CARBIDOPA | C10 H14 N2 O4 | 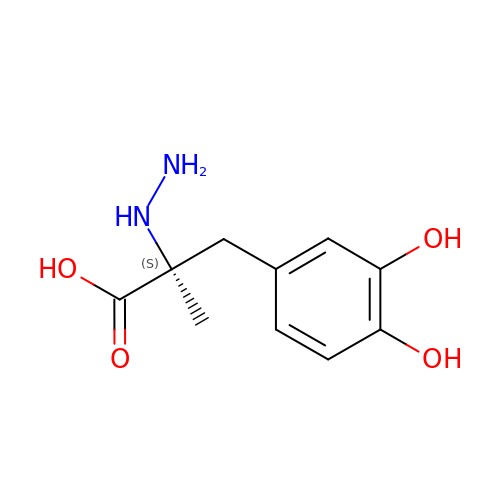TZFNLOMSOLWIDK-JTQLQIEISA-N>[2x]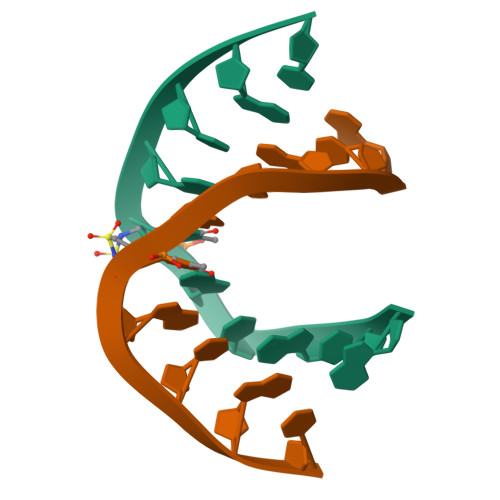GCGTAXACGC Siroheme is the modified isobacteriochlorin tetrapyrrole used by siroheme-dependent sulfite and nitrite reductases (SiR/NiRs) in catalyzing the six-electron reduction of sulfite to sulfide or nitrite to ammonia. CysG is encoded by a gene fusion between a C-terminal SUMT (CysGA) and an N-terminal bifunctional dehydrogenase/ferrochelatase (CysGB). The N-terminal enzyme module, CysGB, is a three-domain bifunctional dehydrogenase/ATP-independent class III ferrochelatase12 that performs the final two steps of siroheme biosynthesis. The C-terminal enzyme module, CysGA, is homologous to a well-studied class of SAM-dependent uro’gen III methyltransferases (SUMTs) that catalyzes the methylations to generate precorrin-210,13.

P1331Cβ sits 3.3 Å below the plane formed by the sirohydrochlorin isobacteriochlorin core, forming a hydrophobic platform for the macrocycle. Both P133G and P133H variants retained the ability to complement the cysG-deficient E. coli when challenged for growth on minimal media, albeit with accumulation of fluorescence indicating altered activity. The P133G variant has 5-fold lower dehydrogenase activity and is about 10-fold lower in its chelatase activity, whereas the P133H variant is deficient for dehydrogenase activity and about 10-fold lower in its chelatase activity. In the P133G-closed active site that binds the tetrapyrrole, the first turn of the α helix from the dimerization domain is unwound, altering the hydrophobic platform on which the evolving substrate sits. The structure of the open active site, as well as the overall fold, is unchanged. Removing the proline platform makes the active site less rigid by unfolding helix 6, presumably impacting its ability to bind and orient the unrestricted precorrin-2 molecule. P133G behaves similarly to D262N: strongly affected by increasing cobalt concentrations.

>MDHLPIFCQLRDRDCLIVGGGDVAERKARLLLEAGARLTVNALTFIPQFTVWANEGMLTLVEGPFDETLLDSCWLAIAATDDDTVNQRVSDAAESRRIFCNVVDAPKAASFIMPSIIDRSPLMVAVSAGGTSGVLARLLREKLESLLPQHLGQVARYAGQLRARVKKQFATMGERRRFWEKFFVNDRLAQSLANADEKAVNATTERLFSEPLDHRGEVVLVGAGPGDAGLLTLKGLQQIQQADIVVYDRLVSDDIMNLVRRDADRVFVGKRAGYHCVPQEEINQILLREAQKGKRVVRLKGGDPFIFGRGGEELETLCHAGIPFSVVPGITAASGCSAYSGIPLTHRDYAQSVRLVTGHLKTGGELDWENLAAEKQTLVFYMGLNQAATIQEKLIAFGMQADMPVALVENGTSVKQRVVHGVLTQLGELAQQVESPALIIVGRVVALRDKLNWFSNH[2x]> SKRKSEAQENIIKNKDELEDFEQGEKYLTLTVSKNDFKKMEVVGQFNLGFIIVTRKVDNKYDLFIVDQHASDEKYNFETLQAVTVFKSQKLIIPQPVELSVIDELVVLDNLPVFEKNGFKLKIDEEEEFGSRVKLLSLPTSKQTLFDLG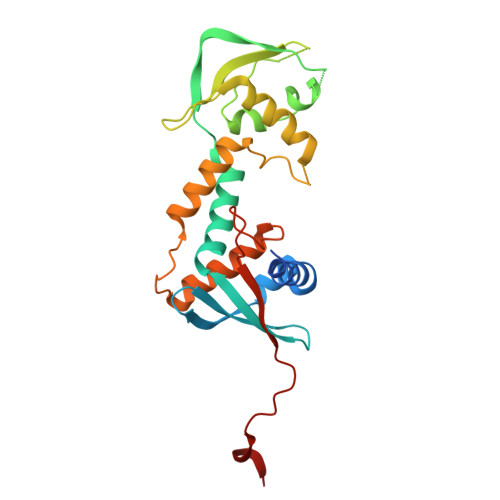DFNELIHLIKEDGGLRRDNIRCSKIRSMFAMRACRSSIMIGKPLNKKTMTRVVHNLSELDKPWNCPHGRPTMRHLMELRDWSSFSKDYEI>MAVVPASLSGQDVGSFAYLTIKDRIPQILTKVIDTLHRHKSEFFEKHGEEGVEAEKKAISLLSKLRNELQTDKPFIPLVEKFVDTDIWNQYLEYQQSLLNESDGKSRWFYSPWLLVECYMYRRIHEAIIQSPPIDYFDVFKESKEQNFYGSQESIIALCTHLQQLIRTIEDLDENQLKDEFFKLLQISLWGNKCDLSLSGGESSSQNTNVLNSLEDLKPFILLNDMEHLWSLLSNCK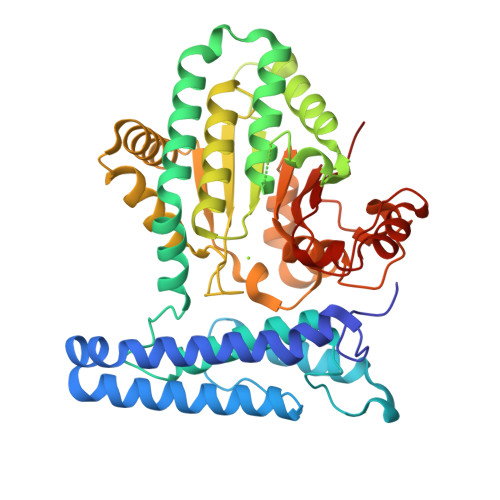KTREKASATRVYIVLDNSGFELVTDLILADFLLSSELATEVHFYGKTIPWFVSDTTIHDFNWLIEQVKHSNHKWMSKCGADWEEYIKMGKWVYHNHIFWTLPHEYCAMPQVAPDLYAELQKAHLILFKGDLNYRKLTGDRKWEFSVPFHQALNGFHPAPLCTIRTLKAEIQVGLQPGQGEQLLASEPSWWTTGKYGIFQYDGPL[2x]> XMNQAIDFAQASIDSYKKHGILEDVIHDTSFQPSGILAVEYSSSAPVAMGNTLPTEKARSKPQFQFTFNKQMQKSVPQANAYVPQDDDLFTLVMTDPDAPSKTDHKWSEFCHLVECDLKLLNEATHETSGATEFFASEFNTKGSNTL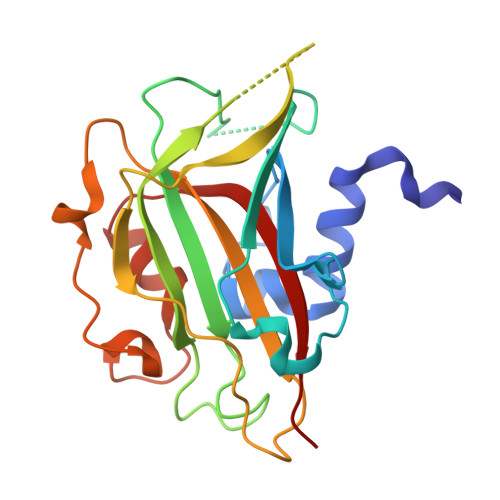IEYMGPAPPKGSGPHRYVFLLYKQPKGVDSSKFSKIKDRPNWGYGTPATGVGKWAKENNLQLVASNFFYAETK>YIFLTPRAYIIVHLLKVGKAKASEISENTQIPYQTVIQNIRWLLAEGYVVKEQKGEEIYYKLTDKGKQMATAELEKIRKLVE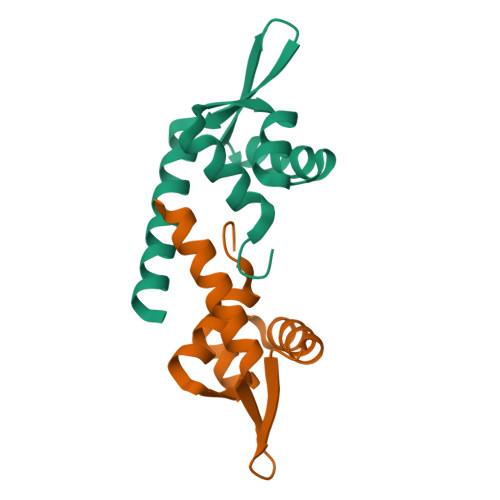VV[2x]>[2x]MEPDLFYILGNKVRRDLLSHLTAMEAYFSLLSSKVSVSSTAVAKHLKIMEREGVLQSYEKEERFIGPTKKYYKISIAKSYVFTLTPEMFWYKGLDLGDAELRDFE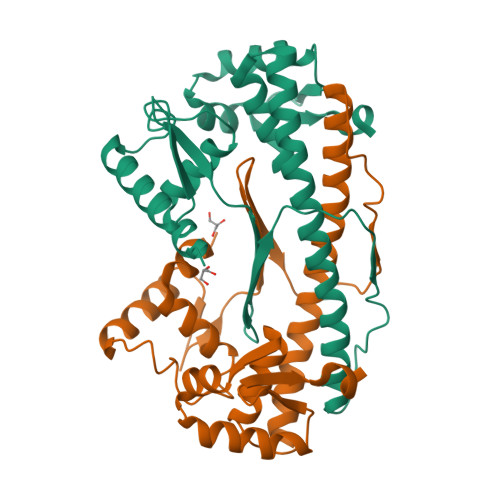ISLSGLDTEPSTLKEMITDFIKANKELEKVLEAFKTIESYRSSLMRKIKEAYLKEIGDMTQLAILHYLLLNGRATVEELSDRLNLKEREVREKISEMARFVPVKIINDNTVVLDEDQILRGEGNEED> SCATGPRNCKDLLDRGYFLSGWHTIYLPDCRPLTVLCDMDTDGGGWTVFQRRMDGSVDFYRDWAAYKQGFGSQLGEFWLGNDNIHALTAQGSSELRVDLVDFEGNHQFAKYKSFKVADEAEKYKLVLGAFVGGSAGNSLTGHNNNFFSTKDQDNDVSSSNCAEKFQGAWWYADCHASNLNGLYLMGPHESFANGINWSAAKGYKY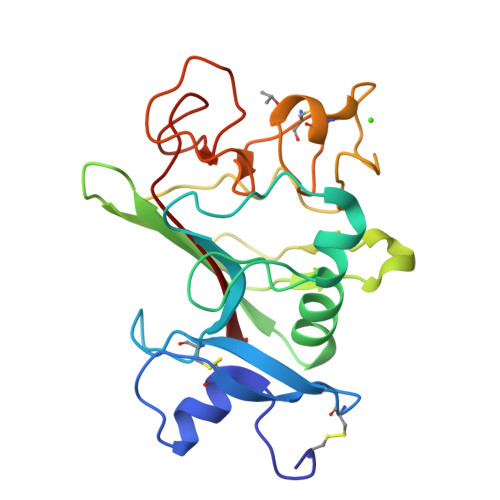SYKVSEMKVRPA>MSDVAETLDPLRLPLQGERLIEASAGTGKTFTIAALYLRLLLGLGGSAAFPRPLTVEELLVVTFTEAATAELRGRIRSNIHELRIACLRETTDNPLYERLLEEIDDKAQAAQWLLLAERQMDEAAVFTIHGFCQRMLNLNAFESGMLFEQQLIEDESLLRYQACADFWRRHCYPLPREIAQVVFETWKGPQALLRDINRYLQGEAPVIKAPPPDDETLASRHAQIVARIDTVKQQWRDAVGELDALIESSGIDRRKFNRSNQAKWIDKISAWAEEETNSYQLPESLEKFSQRFLEDRTKAGGETPRHPLFEAIDQLLAEPLSIRDLVITRALAEIRETVAREKRRRGELGFDDMLSRLDSALRSESGEVLAAAIRTRFPVAMIDEFQDTDPQQYRIFR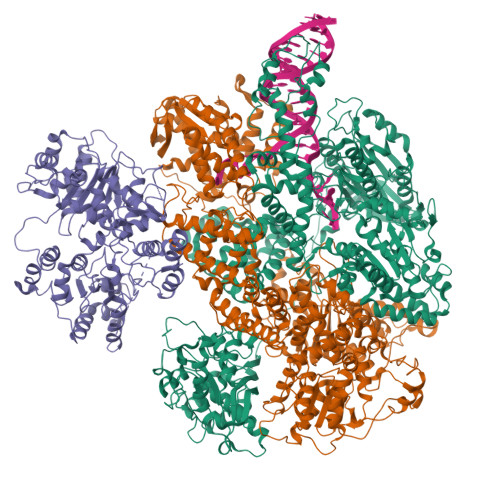RIWHHQPETALLLIGDPKQAIYAFRGADIFTYMKARSEVHAHYTLDTNWRSAPGMVNSVNKLFSQTDDAFMFREIPFIPVKSAGKNQALRFVFKGETQPAMKMWLMEGESCGVGDYQSTMAQVCAAQIRDWLQAGQRGEALLMNGDDARPVRASDISVLVRSRQEAAQVRDALTLLEIPSVYLSNRDSVFETLEAQEMLWLLQAVMTPERENTLRSALATSMMGLNALDIETLNNDEHAWDVVVEEFDGYRQIWRKRGVMPMLRALMSARNIAENLLATAGGERRLTDILHISELLQEAGTQLESEHALVRWLSQHILEPDSNASSQQMRLESDKHLVQIVTIHKSKGLEYPLVWLPFITNFRVQEQAFYHDRHSFEAVLDLNAAPESVDLAEAERLAEDLRLLYVALTRSVWHCSLGVAPLVRRRGDKKGDTDVHQSALGRLLQKGEPQDAAGLRTCIEALCDDDIAWQTAQTGDNQPWQVNDVSTAELNAKTLQRLPGDNWRVTSYSGLQQRGHGIAQDLMPRLDVDAAGVASVVEEPTLTPHQFPRGASPGTFLHSLFEDLDFTQPVDPNWVREKLELGGFESQWEPVLTEWITAVLQAPLNETGVSLSQLSARNKQVEMEFYLPISEPLIASQLDTLIRQFDPLSAGCPPLEFMQVRGMLKGFIDLVFRHEGRYYLLDYKSNWLGEDSSAYTQQAMAAAMQAHRYDLQYQLYTLALHRYLRHRIADYDYEHHFGGVIYLFLRGVDKEHPQQGIYTTRPNAGLIALMDEMFAGMTLEEA[2x];>MLRVYHSNRLDVLEALMEFIVERERLDDPFEPEMILVQSTGMAQWLQMTLSQKFGIAANIDFPLPASFIWDMFVRVLPEIPKESAFNKQSMSWKLMTLLPQLLEREDFTLLRHYLTDDSDKRKLFQLSSKAADLFDQYLVYRPDWLAQWETGHLVEGLGEAQAWQAPLWKALVEYTHQLGQPRWHRANLYQRFIETLESATTCPPGLPSRVFICGISALPPVYLQALQALGKHIEIHLLFTNPCRYYWGDIKDPAYLAKLLTRQRRHSFEDRELPLFRDSENAGQLFNSDGEQDVGNPLLASWGKLGRDYIYLLSDLESSQELDAFVDVTPDNLLHNIQSDILELENRAVAGVNIEEFSRSDNKRPLDPLDSSITFHVCHSPQREVEVLHDRLLAMLEEDPTLTPRDIIVMVADIDSYSPFIQAVFGSAPADRYLPYAISDRRARQSHPVLEAFISLLSLPDSRFVSEDVLALLDVPVLAARFDITEEGLRYLRQWVNESGIRWGIDDDNVRELELPATGQHTWRFGLTRMLLGYAMESAQGEWQSVLPYDESSGLIAELVGHLASLLMQLNIWRRGLAQERPLEEWLPVCRDMLNAFFLPDAETEAAMTLIEQQWQAIIAEGLGAQYGDAVPLSLLRDELAQRLDQERISQRFLAGPVNICTLMPMRSIPFKVVCLLGMNDGVYPRQLAPLGFDLMSQKPKRGDRSRRDDDRYLFLEALISAQQKLYISYIGRSIQDNSERFPSVLVQELIDYIGQSHYLPGDEALNCDESEARVKAHLTCLHTRMPFDPQNYQPGERQSYAREWLPAASQAGKAHSEFVQPLPFTLPETVPLETLQRFWAHPVRAFFQMRLQVNFRTEDSEIPDTEPFILEGLSRYQINQQLLNALVEQDDAERLFRRFRAAGDLPYGAFGEIFWETQCQEMQQLADRVIACRQPGQSMEIDLACNGVQITGWLPQVQPDGLLRWRPSLLSVAQGMQLWLEHLVYCASGGNGESRLFLRKDGEWRFPPLAAEQALHYLSQLIEGYREGMSAPLLVLPESGGAWLKTCYDAQNDAMLDDDSTLQKARTKFLQAYEGNMMVRGEGDDIWYQRLWRQLTPETMEAIVEQSQRFLLPLFRFNQS[2x];>MKLQKQLLEAVEHKQLRPLDVQFALTVAGDEHPAVTLAAALLSHDAGEGHVCLPLSRLENNEASHPLLATCVSEIGELQNWEECLLASQAVSRGDEPTPMILCGDRLYLNRMWCNERTVARFFNEVNHAIEVDEALLAQTLDKLFPVSDEINWQKVAAAVALTRRISVISGGPGTGKTTTVAKLLAALIQMADGERCRIRLAAPTGKAAARLTESLGKALRQLPLTDEQKKRIPEDASTLHRLLGAQPGSQRLRHHAGNPLHLDVLVVDEASMIDLPMMSRLIDALPDHARVIFLGDRDQLASVEAGAVLGDICAYANAGFTAERARQLSRLTGTHVPAGTGTEAASLRDSLCLLQKSYRFGSDSGIGQLAAAINRGDKTAVKTVFQQDFTDIEKRLLQSGEDYIAMLEEALAGYGRYLDLLQARAEPDLIIQAFNEYQLLCALREGPFGVAGLNERIEQFMQQKRKIHRHPHSRWYEGRPVMIARNDSALGLFNGDIGIALDRGQGTRVWFAMPDGNIKSVQPSRLPEHETTWAMTVHKSQGSEFDHAALILPSQRTPVVTRELVYTAVTRARRRLSLYADERILSAAIATRTERRSGLAALFSSRE[2x]>[2x]STAGKVIKCKAAVLWEEKKPFSIEEVEVAPPKAHEVRIKMVATGICRSDDHVVSGTLVTPLPVIAGHEAAGIVESIGEGVTTVRPGDKVIPLWTPQCGKCRVCKHPEGNFCLKNDLSMPRGTMQDGTSRFTCRGKPIHHFLGTSTFSQYTVVDEISVAKIDAASPLEKVCLIGCGFSTGYGSAVKVAKVTQGSTCAVFGLGGVGLSVIMGCKAAGAARIIGVDINKDKFAKAKEVGATECVNPQDY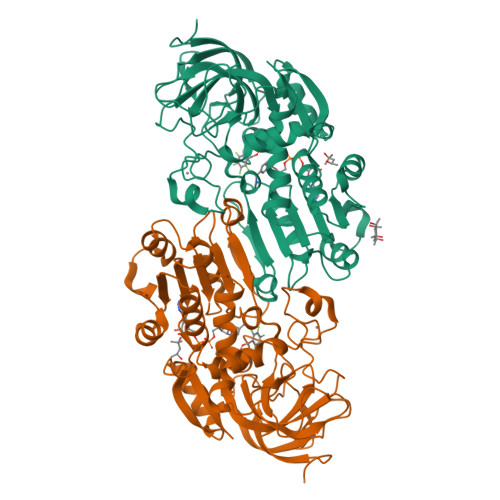KKPIQEVLTEMSNGGVDFSFEVIGRLDTMVTALSCCQEAYGVSVIVGVPPDSQNLSMNPMLLLSGRTWKGAIFGGFKSKDSVPKLVADFMAKKFALDPLITHVLPFEKINEGFDLLRSGESIRTILTF> MVECITPEAIFIGANKQTQVSDIHKVKKIVAFGAGKTIALWDPIEPNNKGVYATLKGHEAEVTCVRFVPDSDFMVSASEDHHVKIWKFTDYSHLQCIQTIQHYSKTIVALSALPSLISVGCADGTISIWRQNIQNDEFGLAHEFTIKKGFFYPLCLSLSKVEEKKYLLAIGGTNVNVFIASFILSDSGIEKCRVVAELEGHEDWVKSLAFRHQETPGDYLLCSGSQDRYIRLWRIRINDLIDDSEEDSKKLTLLSNKQYKFQIDDELRVGINFEALIMGHDDWISSLQWHESRLQLLAATADTSLMVWEPDETSGIWVCSLRLGEMSSKGASTATGSSGGFWSCLWFTHERMDFFLTNGKTGSWRMWATKDNIICDQRLGISGATKDVTDIAWSPSGEYLLATSLDQTTRLFAPWIYDASGRKREIATWHEFSRPQIHGYDMICVETVTDTRFVSGGDEKILRSFDLPKGVAGMLQKFVGIQFEEKSEMPDSATVPVLGLSNKAGEDDANEDDEEEEGGNKETPDITDPLSLLECPPMEDQLQRHLLWPEVEKLYGHGFEITCLDISPDQKLIASACRSNNVQNAVIRIFSTENWLEIKPALPFHSLTITRLKFSKDGKFLLSVCRDRKWALWERNMEDNTFELRFKNEKPHTRIIWDADWAPLEFGNVFVTASRDKTVKVWRHQKEPADDYVLEASIKHTKAVTAISIHDSMIREKILISVGLENGEIYLYSYTLGKFELITQLNEDITPADKITRLRWSHLKRNGKLFLGVGSSDLSTRIYSLAYE

The highly conserved eukaryotic Elongator complex performs specific chemical modifications on wobble base uridines of tRNAs, which are essential for proteome stability and homeostasis. The complex is formed by six individual subunits (Elp1‐6) that are all equally important for its tRNA modification activity. Here, we report the structures of the fully assembled yeast Elongator and the Elp123 sub‐complex solved by an integrative structure determination approach showing that two copies of the Elp1, Elp2, and Elp3 subunits form a two‐lobed scaffold, which binds Elp456 asymmetrically. The eukaryotic Elongator complex has been associated with a plethora of cellular activities 8, 9, 10, but nowadays, it is widely accepted that the main cellular function of the Elongator complex is the formation of 5‐methoxycarbonylmethyl‐uridine (mcm5U), 5‐methoxycarbonylmethyl‐2‐thio‐uridine (mcm5s2U), and 5‐carbamoylmethyl‐uridine (ncm5U) in the wobble base position of 11 eukaryotic tRNAs 10.

A difference map between the full Elp123 model and the asymmetric model rendered, apart from a minor difference in the bottom part, a bean‐shaped density (Fig EV4E). Our group also independently solved the yeast Elp2 structure at 2.8 Å resolution (Appendix Table S1 and Fig EV4F), which is highly similar (r.m.s.d. = 1.19 Å686Cα) to the previously published Elp2 structure 30. In summary, the presented 3D models allow us to position the CTD of Elp1 within the arch and the Elp2 within the wings, though the precise orientation of Elp2 is still unclear. The orientation of Elp2 in the wing of the map is restrained by crosslinks from the N‐terminal WD40 domain of Elp2 to Elp1‐CTD and the N‐terminus of Elp3. Elp2 is located peripherally attached to Elp1‐CTD and Elp3. In detail, the active site of Elp3 is located in the conserved cavity formed by Elp3, the N‐terminal WD40 domain of Elp2, and the α‐solenoid domain of Elp1‐CTD. The region of Elp2 contributing to the cavity includes residues 201–204, which were found to be important for tRNA modification activity of Elongator. Finally, to understand the contribution of individual conserved surface residues in Elp2, we mutated residues in the previously identified 30 basic region (R626, R628, R654, R675), which was described to be important for histone acetylation and microtubule binding. Although we show that mutating the residues of this patch (R626, R628, R654, R675) affects Elongator's activity, it is not involved in protein–protein interactions within the Elp123 sub‐complex. None of the tested mutations affects the stability of Elp2 (Fig EV5C) and we therefore believe that these regions are involved in protein–protein interactions.(1~{Z})-1-(3-ethyl-5-methoxy-1,3-benzothiazol-2-ylidene)propan-2-one | C13 H15 N O2 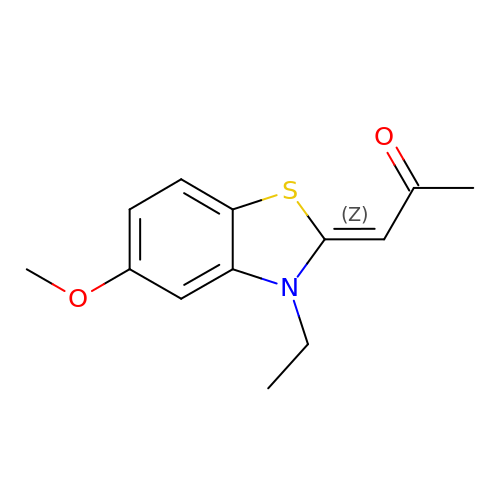S | BGVLELSCIHASRV-QPEQYQDCSA-N> E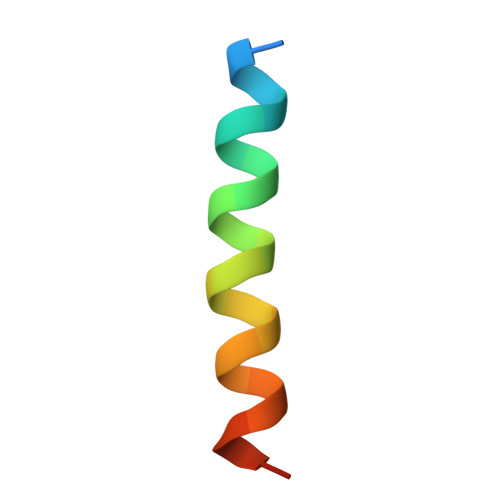ARTEVQIARKLQCIADQFHRLHIQR> GDAASDLKSRLDKVSSFHASFTQKVTDGSGAAVQEGQGDLWVKRPNLFNWHMTQPDESILVSDGKTLWFY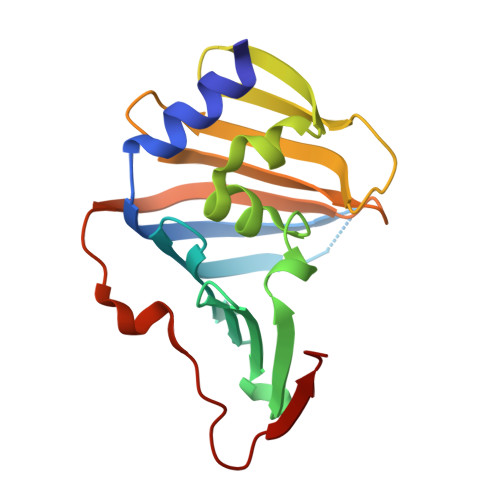NPFVEQATATWLKDATGNTPFMLIARNQSSDWQQYNIKQNGDDFVLTPKASNGNLKQFTINVGRDGTIHQFSAVEQDDQRSSYQLKSQQNGAVDAAKFTFTPPQGVTVDDQRK>[2x]SGPKKYFPIPVE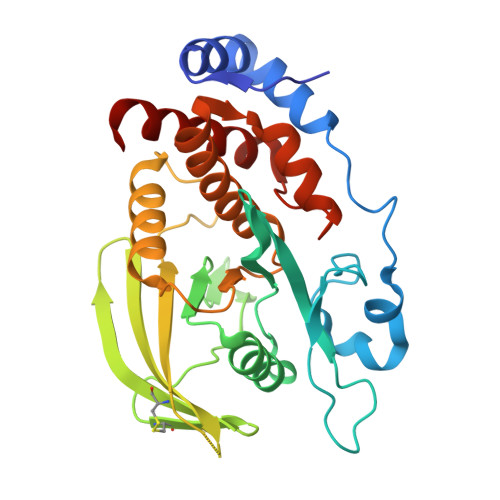HLEEEIRIRSADDCKQFREEFNSLPSGHIQGTFELANKEENREKNRYPNILPNDHSRVILSQLDGIPCSDYINASYIDGYKEKNKFIAAQGPKQETVNDFWRMVWEQKSATIVMLTNLKERKEEKCHQYWPDQGCWTYGNIRVCVEDCVVLVDYTIRKFCIQPQLPDGCKAPRLVSQLHFTSWPDFGVPFTPIGMLKFLKKVKTLNPVHAGPIVVHCSAGVGRTGTFIVIDAMMAMMHAEQKVDVFEFVSRIRNQRPQMVQTDMQYTFIYQALLEYYLYG>[3x]ARASPGSAASPRLREGPELSPDDPAGLLDLRQGMFAQLVAQNVLLIDGPLSWYSDPGLAGVSLTGGLSYKEDTKELVVAKAGVYYVFFQLELRRVVAGEGSG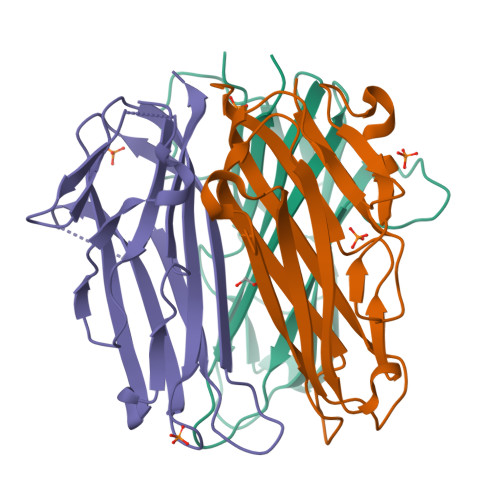SVSLALHLQPLRSAAGAAALALTVDLPPASSEARNSAFGFQGRLLHLSAGQRLGVHLHTEARARHAWQLTQGATVLGLFRVTPEIPAGLPSPRSEGSHHHHHHHH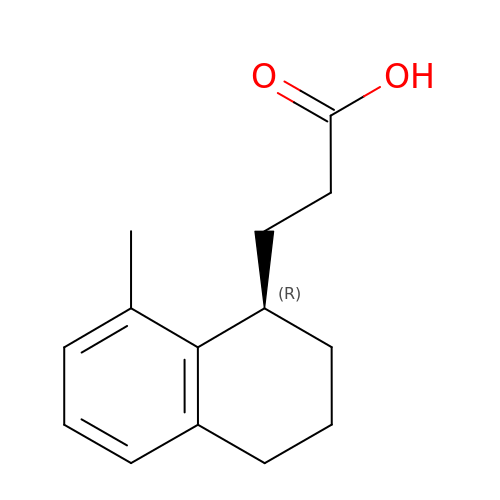3-[(1R)-8-methyl-1,2,3,4-tetrahydronaphthalen-1-yl]propanoic acid | C14 H18 O2 | IAGVZFLDKNPTAP-GFCCVEGCSA-N> MGAGGFRKNTGRNNTTLPYN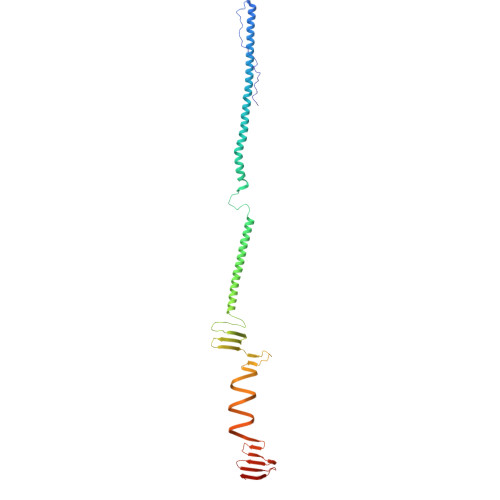VGFLNNVQDTETYNVAVYDELQKVSTATNQMFQAIDEIHEEIDVRIKALNAMNLQFDELENRITTEIETAIADIQTQMGNLSTEDIWDNSVQPPVKLESTVSGFKTSIEGNTTKIQTVEGIVNDQGQEIALVQTELQNINGSLSQYMKLSEYEATWGVNSTVNGRYAGVKLTNNGTNSQFQVTANKFIVGDGSSGNTPFVFEGGRARMEFADIKNVNITTAQIANARIQWAQIDNVSISNAQIQNLSADKITAGSMWGSNWRLTVGGDFVMGGTGGAQLWMNGNRIDFYDGSGALRIRIGSW> TLKLCSPEEFTRLCREKTQEIYPIKEANGRTRKALIICNTEFKHLSLRYGANFDIIGMKGLLEDLGYDVVVKEELTAEGMESEMKDFAALSEHQTSDSTFLVLMSHGTLHGICGTMHSEKTPDVLQYD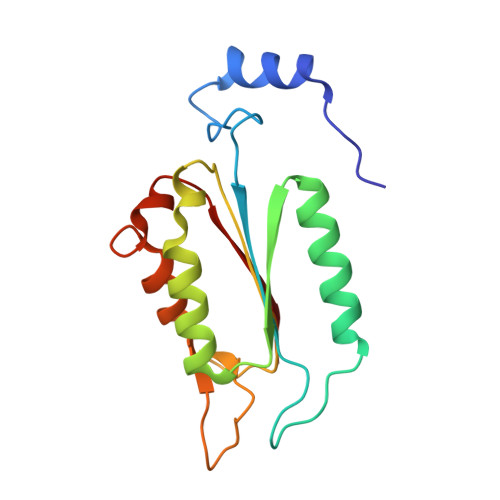TIYQIFNNCHCPGLRDKPKVIIVQAA> MAHHHHHHSAALEVLFQGPGSGCYTYQVSRHSTEMLHNLNQQRKNGGRFCDVLLRVGDESFPAHRAVLAACSEYFESVFSAQLGDGGAADGGPADVGGAAAAPGGGAGGSRELEMHTISSKVFGDILDFAYTSRIVVRLESFPELMTAAKFLLMRSVIEICQEVI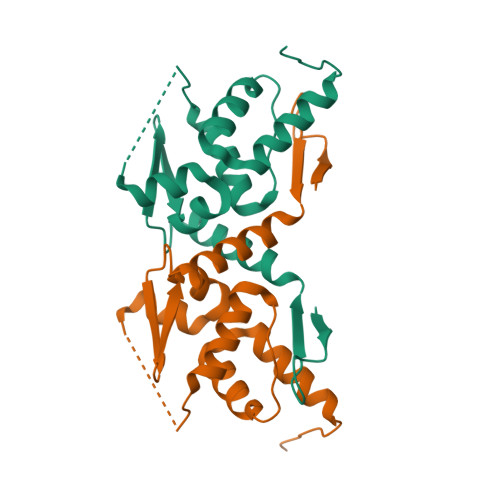KQSNVQILVP>[2x]HHHHHHPCCSNPCQNRGECMSTGFDQYKCDCTRTGFYGENCTTPEFLTRIKLLLKPTPNTVHYILTHFKGVWNIVNNIPFLRSLIMKYVLTSRSYLIDSPPTYNVHYGYKSWEAFSNLSYYTRALPPVADDCPTPMGVKGNKELPDSKEVLEKVLLRREFIPDPQGSNMMFAFF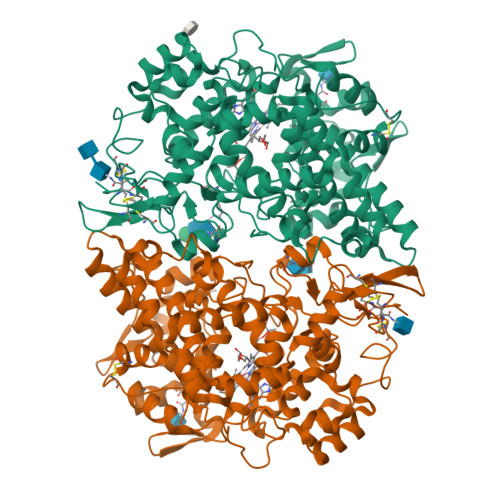AQHFTHQFFKTDHKRGPGFTRGLGHGVDLNHIYGETLDRQHKLRLFKDGKLKYQVIGGEVYPPTVKDTQVEMIYPPHIPENLQFAVGQEVFGLVPGLMMYATIWLREHNRVCDILKQEHPEWGDEQLFQTSRLILIGETIKIVIEDYVQHLSGYHFKLKFDPELLFNQQFQYQNRIASEFNTLYHWHPLLPDTFNIEDQEYSFKQFLYNNSILLEHGLTQFVESFTRQIAGRVAGGRNVPIAVQAVAKASIDQSREMKYQSLNEYRKRFSLKPYTSFEELTGEKEMAAELKALYSDIDVMELYPALLVEKPRPDAIFGETMVELGAPFTLKGLMGNPICSPQYWKPSTFGGEVGFKIINTASIQSLICNNVKGCPFTSFNVQDPQPTKTATIAASASHSRLDDINPTVLIKRRSTEL>[6x]KLTKEELKEIVTMMVNKLTNRLSEQNINIIVTDKAKDKIAEEGYDPEYGARPLIRAIQKTIEDNLSELILDGNQIEGKKVTV;>LTKINETESEKLLSLEDTLHERVIGQKDAVNSISKAVRRARAGLKDPKRPIGSFIFLGPTGVGKTELARALAESMFGDDDAMIRVDMSEFMEKHAVSRLVGAPPGYVGHDDGGQLTEKVRRKPYSVILFDEIEKAHPDVFNILLQVLDDGHLTDTKGRTVDFRNTIIIMTSNVGAQELQDQRFAGFGGSSDGQDYETIRKTMLKELKNSFRPEFLNRVDDIIVFH[6x];>NNLKEIEQEIEKVKNEKDAAVHAQEFENAANLRDKQTKLEKQYEEAKNEWKNAQN[6x];>SVVDTVAILKGLRDRYEAHHRINISDEAIEAAVKLSNRYVSDRFLPDKAIDLIDEASSKVRLKSHTTPNNLKEIEQEIEKVKNEKDAAVHAQEFENAANLRDKQTKLEKQYEEAKNEWKNAQNGMSTSLSEEDIAEVIAGWTGIP[6x];>[6x]TLDSLARDLTVIAKDGTLDPVIGRDKEITRVIEVLSRRTKNNPVLIGEPGVGKTAIAEGLAQAIVNNEVPETLKDKRVMSLDMGTVVAGTKYRGEFEERLKKVMEEIQQAGNVILFIDELHTLVGAGGAEGAIDASNILKPALARGELQCIGATTLDEYRKNIEKDAALERRFQPVQVDEP;>RLTERAQRVLAHAQEEAIRLNHSNIGTEHLLLGLMKEPEGIAAKVLESFNITEDKVIEEVEKLIGHGQDHVGTLHYTPRAKKVIELSMDEARKLHHNFVGTEHILLGLIRENEGVAARVFANLDLNITKARAQVVKALGNPEMSNKNAQASKSNNTP[6x];>MRIERVDDTTVKLFITYSDIEARGFSREDLWTNRKRGEEFFWSMMDEINEEEDFVVEGPLWIQVHAFEKGVEVTISKSKNEDMMNMSDDD[6x]

The bacterial AAA+ chaperone ClpC associates with the peptidase ClpP to form a central proteolytic machinery of Gram-positive bacteria. The ClpC-ClpP machinery acts in regulatory and general proteolysis, controlling multiple cellular pathways and differentiation processes and is crucial for bacterial stress resistance and virulence. ClpC activity crucially relies on cooperation with adaptor proteins including MecA, that target specific substrates while concurrently stimulating ClpC ATPase activity. Here, we report on an unexpected mode of AAA+ chaperone control involving transition between an inactive resting state and a functional hexamer as revealed by determining the cryoEM-structures of S. aureus ClpC in absence and presence of MecA.

Additional extra density caps the hexamer and accounts for the N-terminal domain of MecA, whose structure is unknown. MecA binds to N-terminal and middle domains of each ClpC subunit forming a separate layer on top of the ClpC AAA ring. Additionally, binding of MecA to MDs breaks head-to-head MD contacts and is therefore expected to prevent formation of the ClpC resting state. MecA prevents MD interactions and thereby converts ClpC into a canonical and active hexamer. Taken together, our structures of ClpC alone or in complex with MecA show a dramatic reorganization from a helical resting state to a planar canonical AAA+ hexamer, explaining ClpC activation by the adaptor MecA. Quantification of co-eluting MecA suggests the formation of a 1:1 ClpC:MecA complex, consistent with the binding stoichiometry determined for B. subtilis ClpC/MecA complexes and mass determination by SLS (767 kDa). This indicates that MecA binding shifts ClpC from a large, non-hexameric assembly to a ClpC6/MecA6 complex. Once formed the hexameric ClpC6/MecA6 complex is stable and does not dissociate spontaneously, raising the question how ClpC activation is turned off.>SNAVGQFANFVDLLQYRAKLQARKTVFSFLADGEAESAALTYGELDQKAQAIAAFLQANQAQGQRALLLYPPGLEFIGAFLGCLYAGVVAVPAYPPRPNKSFDRLHSIIQDAQAKFALTTTELKDKIADRLEALEGTDFHCLATDQVELISGKNWQKPNISGTDLAFLQYTSGSTGDPKGVMVSHHNLIHNSGLINQGFQDTEASMGVSWLPPYHDMGLIGGILQ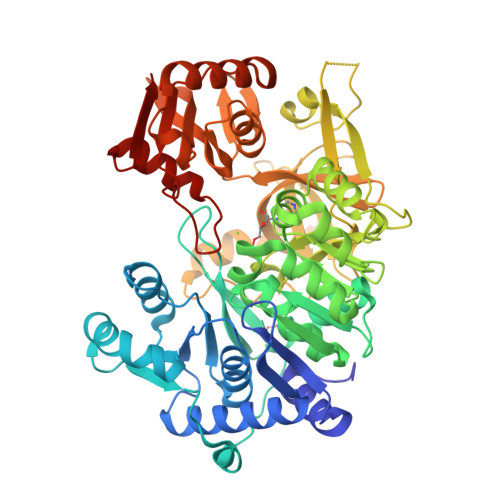PIYVGATQILMPPVAFLQRPFRWLKAINDYRVSTSGAPNFAYDLCASQITPEQIRELDLSCWRLAFSGAEPIRAVTLENFAKTFATAGFQKSAFYPCYGMAETTLIVSGGNGRAQLPQEIIVSKQGIEANQVRPAQGTETTVTLVGSGEVIGDQIVKIVDPQALTECTVGEIGEVWVKGESVAQGYWQKPDLTQQQFQGNVGAETGFLRTGDLGFLQGGELYITGRLKDLLIIRGRNHYPQDIELTVEVAHPALRQGAGAAVSVDVNGEEQLVIVQEVERKYARKLNVAAVAQAIRGAIAAEHQLQPQAICFIKPGSIPKTSSGKIRRHACKAGFLDGSLAVVGEWQ[2x]>[2x]AD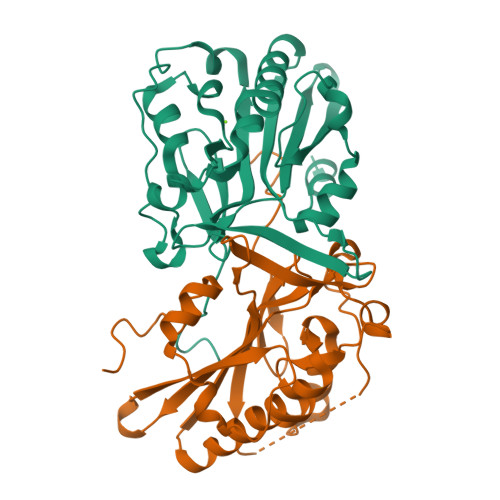LPALPGGPAGGTGELAKYGLPGVAQLRSRESYVLSYDPRTRGALWVLEQLRPERLRGDGDRSAADFREDDSVHAYHRATNADYRGSGFDRGALAAAANHRWSQRAMDDTFYLSNVAPQVPHLNQNAWNNLERYSRSLTRTYQNVYVCTGPLFLPRTEADGKSYVKYQVIGKNHVAVPTHFFKVLILEAAGGQIELRSYVMPNAPVDETIPLERFLVPIESIERASGLLFVPNILARAGNLKAITAGS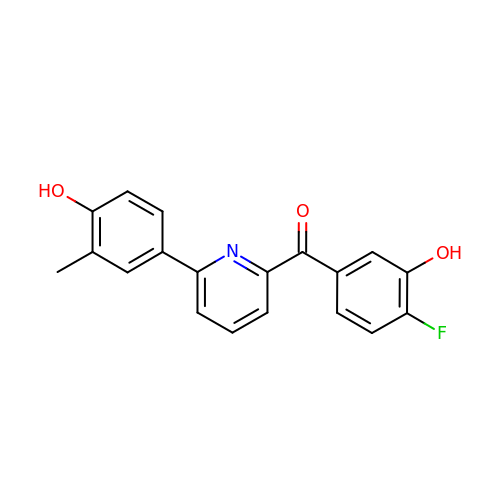(4-fluoranyl-3-oxidanyl-phenyl)-[6-(3-methyl-4-oxidanyl-phenyl)pyridin-2-yl]methanone | C19 H14 F N O3 | QDDLZOOWBSJEFI-UHFFFAOYSA-N Among these, the adhesion of UPECs to the host uroepithelial tissues is due to the E. coli type 1 pili, called FimH, which mediate their attachment in a mannose-dependent interaction. FimH adhesin of type 1 fimbriae promotes intestinal colonization by binding to colonic crypts of epithelial cells, facilitating E. coli adhesion and invasion to the urinary epithelium, a key player in UPEC pathogenicity. Importantly, the mannose-specific adhesin FimH has an essential hydrophobic binding pocket of non-polar amino acids that surrounds the aglycon portion of α-D-mannopyranoside glycomimetics. Preventing bacterial FimH adhesion to highly mannosylated glycoprotein uroplakin Ia from bladder cells represents an appealing strategy to control UTIs.

The crystal structure of the FimH lectin-binding domain co-crystallized with inhibitor 11 was obtained at a resolution of 3 Å. Delightfully, the co-crystal structure of compound 11 and E. coli C43 (DE3) FimH also revealed the expected 4C1 chair conformation of the ligand 11 bound into the active site of the tyrosine gate. In the mannose-binding site of FimH, we observed Tyr48 in parallel, while the Tyr137 residue was in T-aromatic stacking with the quinoline group of ligand 11. Four FimH lectin domains were observed in the asymmetric unit of the crystal and the mannose-binding site of each FimH lectin domain was in proximity with a symmetry-related neighbor in the crystal packing. The two binding sites of FimH molecules were held together by the two quinoline substituents crossed over in a parallel stacking, while their mannosides projected into the binding pocket of FimH. Therefore, the binding of FimH to compound 11 appeared to simulate the bivalent binding of the natural oligomannosidic N-glycan structures. Inhibitor 11 interacted via different amino acids that included Ile 13, Phe 1, Asp 47, Gln 133, Asp 54, Asn 135, Asp 140, Phe 142 in the open conformation of FimH. Interestingly, the inter-molecular π-π stacking of two quinolines residues of 11 triggered the interlacing of two FimH lectins, providing a “bidentate’’ complex. Interestingly, among the mannosides studied, the quinoline analog 11, having an IC50 of 3.17 nM, was the most efficient at reducing FimH-mediated bacterial adherence. Although compound 20 had a higher inhibitory potency (IC50 0.82 ± 0.4) against isolated FimH lectin binding domain, ligand 11 (IC50 3.17 ± 2.3) showed better potency in inhibiting bacterial adhesion to bladder HTB-9 cell monolayers without adverse side effects.

>[4x]FACKTANGTAIPIGGGSANVYVNLAPVVNVGQNLVVDLSTQIFCHNDYPETITDYVTLQRGSAYGGVLSNFSGTVKYSGSSYPFPTTSETPRVVYNSRTDKPWPVALYLTPVSSAGGVAIKAGSLIAVLILRQTNNYNSDDFQFVWNIYANNDVVVPT>MGHHHHHHLESTSLYKKSSSTPPRGVTVVNNFDCKRYLGTWYEIARFDHRFERGLEKVTATYSLRD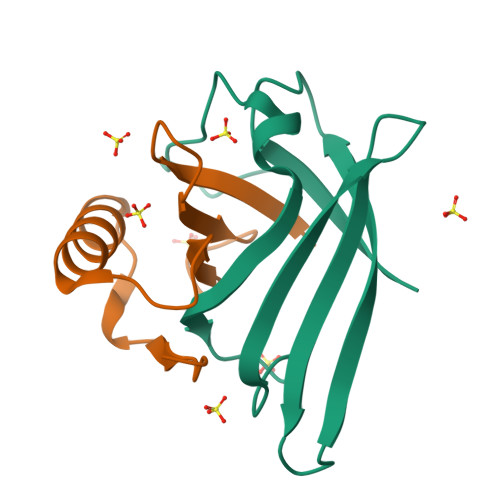DGGLNVINKGYNPDRGMWQQSEGKAYFTGAPTRAALKVSFF[3x];>[3x]MGPFYGGYNVIALDREYRHALVCGPDRDYLWILSRTPTISDEVKQEMLAVATREGFDVSKFIWVQQPGS> MQQKSDNVVSHYVFEAPVRIWHWLTVLCMAVLMVTGYFIGKPLPSVSGEATYLFYMGYIRLIHFSAGMVFTVVLLMRIYWAFVGNRYSRELFIVPVWRKSWWQGVWYEIRWYLFLAKRPSADIGHNPIAQAAMFGYFLMSVFMIITGFALYSEHSQYAIFAPFRYVVEFFYWTGGNSMDIHSWHRLGMWLIGAFVIGHVYMALREDIMSDDTVI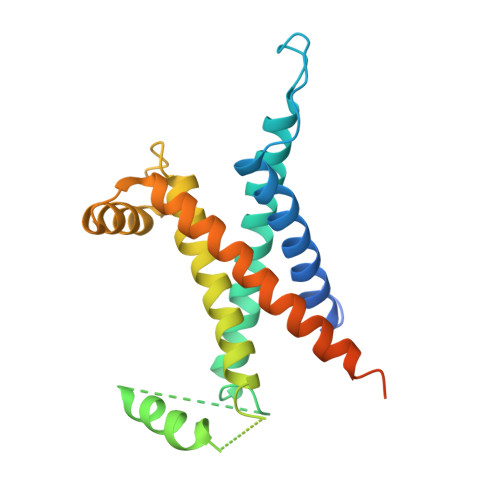STMVNGYRSHKFGKISNKERS> MAFKGQPTPSTITQITRAKISDG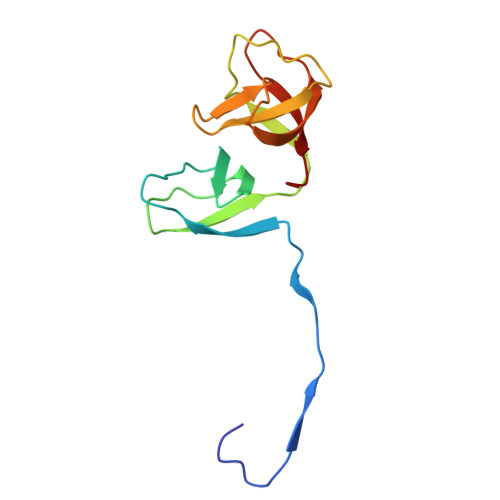KSVRVILSEGESTKTQQFYLINGFFGVAMQDGEKGDEVTLQIEQAEYETDNIVTSEAFEAGKLIYWDNTAKKFTTTSASNRLVGRVTDGKDSNNVIWFILLPQQ>SELSFNYPNFQSVEDITFQGGASPRNETLQLTPTDSNGIPIRQRAGHAVYSQPFQLRDTSFYTTFTFVIRTTSNSPADGFAIFIAPPDFPVKRYGGYLGLFEPNTATNTSANKVVAVEFDTWVNTEWKEPRYRHIGIDVNSIVSVRVTRWQDKDV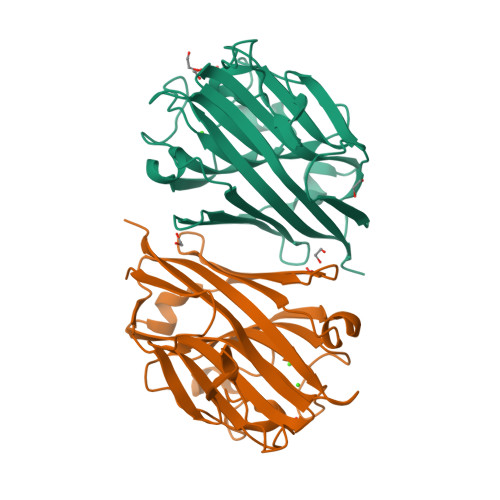FSRSIATAHVGYDGISKILTAFVTYPDGGNYVLSHVVDLAEIFPGDVRIGFSGATGQYETQYIHSWSFSSTSTNLLRDGARHHHHHH[2x]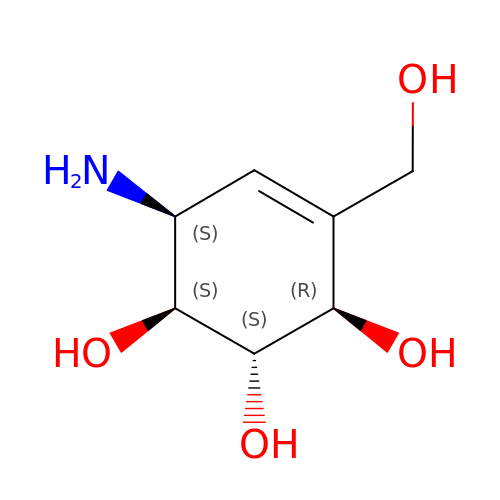6-AMINO-4-HYDROXYMETHYL-CYCLOHEX-4-ENE-1,2,3-TRIOL | C7 H13 N O4 | XPHOBMULWMGEBA-VZFHVOOUSA-N>MESSTQTKPGSLIVVGTGIESIGQMTLQALSYIEAASKVFYCVIDPATEAFILTKNKNCVDLYQYYDNGKSRMDTYTQMAELMLKEVRNGLDVVGVFYGHPGVFVNPSHRALAIARSEGYQARMLPGVSAEDCLFADLCIDPSNPGCLTYEASDFLIRERPVNVHSHLILFQVGCVGIADFNFSGFDNSKFTILVDRLEQEYGPDHTVVHYIAAMMPHQDPVTDKFTIGQLREPEIAKRVGGVSTFYIPPKARKDINTDIIRLLEFLPAGKVPDKHTQIYPPNQWEPDVPTLPPYGQNEQAAITRLEAHAPPEEYQPLATSKAMTDVMTKLALDPKALAEYKADHR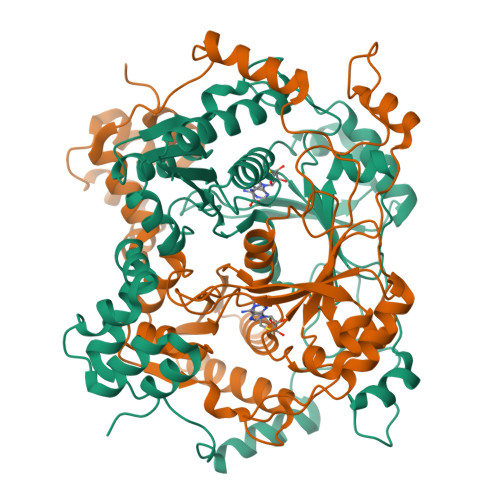AFAQSVPDLTPQERAALELGDSWAIRCAMKNMPSSLLEAA[6x]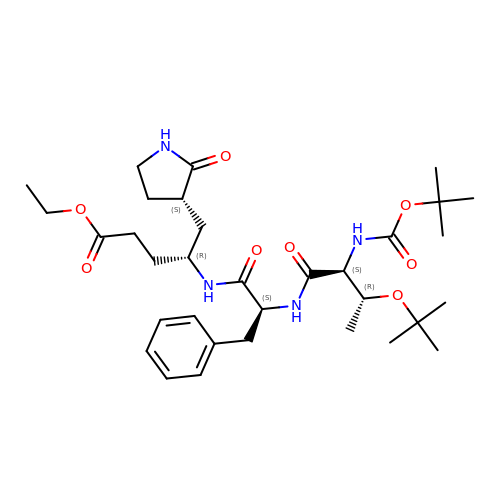N-(tert-butoxycarbonyl)-O-tert-butyl-L-threonyl-N-{(2R)-5-ethoxy-5-oxo-1-[(3S)-2-oxopyrrolidin-3-yl]pentan-2-yl}-L-phenylalaninamide | C33 H52 N4 O8 | SNZMLKYHPQYHPN-DPURIWRLSA-N3-methyl-8-((8-methyl-8-azabicyclooctan-3-yl)amino)-1,7-naphthyridin-2(1H)-one 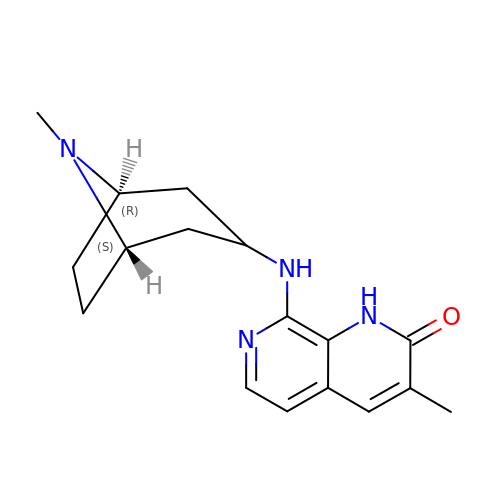| C17 H22 N4 O | HBGWEOSHQILMON-ZSOGYDGISA-N>MTDVIKPDYLEYDDLLDRDEMFTILEEYFMYRGLLGLRIKYGRLFNEIKKFDNDAEEQFGTIEELKQKLRLNSEEGADNFIDYIKVQKQDIVKL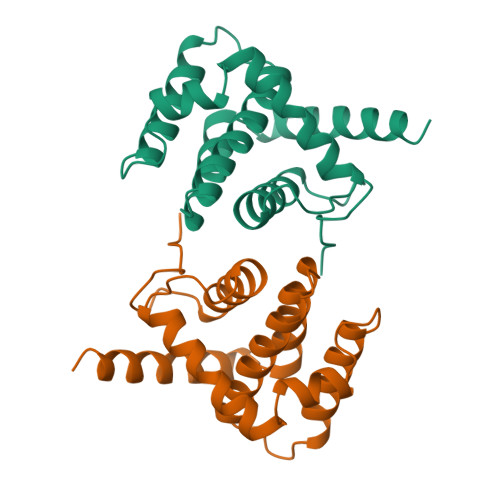TVYDCISMIGLCACVVDVWRNEKLFSRWKYCLRAIKLFINDHMLDKIKSILQNRLVYVEMSKHHHHHH[2x]> MLINNKKLLHHILPILVLALLGMRTAQAVAPGIVIPPKALFTQQGGAYGRCPNGTRALTVAELRGN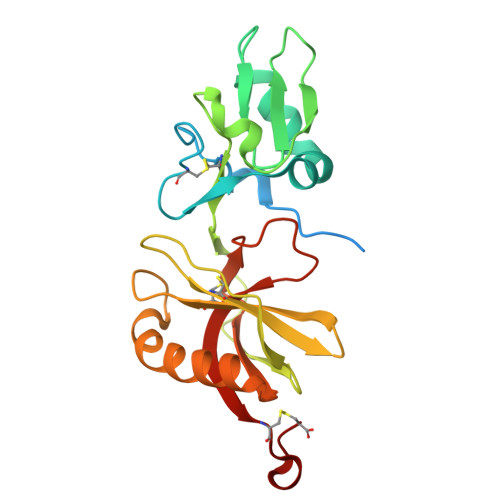AELQTYLRQITPGWSIYGLYDGTYLGQAYGGIIKDAPPGAGFIYRETFCITTIYKTGQPAADHYYSKVTATRLLASTNSRLCAVFVRDGQSVIGACASPYEGRYRDMYDALRRLLYMIYMSGLAVRVHVSKEEQYYDYEDATFQTYALTGISLCNPAASIC7-[3-(aminomethyl)-4-(cyclopropylmethoxy)phenyl]-4-methylquinolin-2-amine 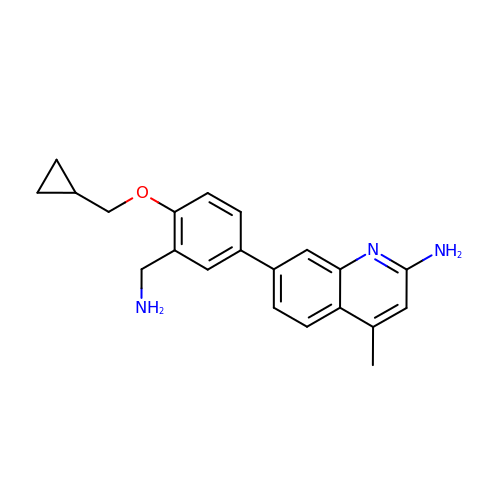| C21 H23 N3 O | YJCSKOOAQMAARS-UHFFFAOYSA-N> MAKLTALTLLGMGLALFDRQKSSFQTRFNVHREVTPVELPNCNLVKGIDNGSEDLEILPNGLAFISSGLKYPGIMSFDPDKSGKILLMDLNEKEPAVSELEIIGNTLDISSFNPWGISTFIDDDNTVYLLVVNHPGSSSTVEVFKFQEEEKSLLHLKTIRHKLLPSVNDIVAVGPEHFYATNDHYFIDPYLKSWEMHLGLAWSFVTYYSPNDVRVVAEGFDFANGINISPDGK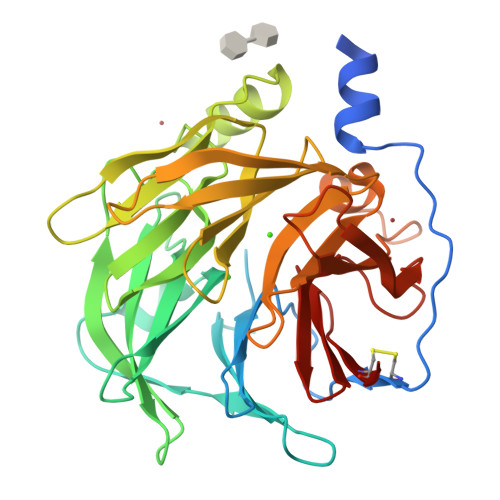YVYIAELLAHKIHVYEKHANWTLTPLRVLSFDTLVDNISVDPVTGDLWVGCHPNGMRIFFYDAENPPGSEVLRIQDILSEEPKVTVVYAENGTVLQGSTVAAVYKGKLLIGTVFHKALYCDL> MNKHTNLVTSSFNLTKPMKSFIRRNGLR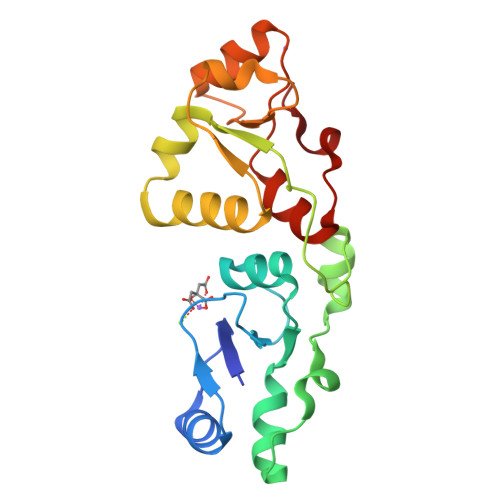VQESVTDETDFVILGSPPLRRTHKFLLATSLGIPLVSSQYLTDCIKSGKVLDFRSYKYKDEEAEAKWGFRLDDIHRRTCFNGKRLYITKAIRDSMVGDSIHGLYSILETSGAEIVGDIKRAQEKDTIILAQPDNDQEGRNMSATGLNVYKIELVALSILRDRIDFDEFLID> MAHHHHHHMDVGELLSYQPNRGTKRPRDDEEEEQKMRRKQTGTRERGRYREEEMTVVEEADDDKKRLLQIIDRDGEEEEEEEEPLDESSVKKMILTFEKRSYKNQELRIKFPDNPEKFMESELDLNDIIQEMHVVATMPDLYHLLVELNAVQSLLGLLGHDNTDVSIAVVDLLQELTDIDTLHESEEGAEVLIDALVDGQVVALLVQNLERLDESVKEEADGVHNTLAIVENMAEFRPEMCTEGAQQGLLQWLLKRLKAKMPFDANKLYCSEVLAILLQDNDENRELLGELDGIDVLLQQLSVFKRHNPSTAEEQEMMENLFDSLCSCLMLSSNRERFLKGEGLQLMNLMLREKKISRSSALKVLDHAMIGPEGTDNCHKFVDILGLRTIFPLFMKSPRKIKKVGTTEKEHEEHVCSILASLLRNLRGQQRTRLLNKFTENDSEKVDRLMELHFKYLGAMQVADKKIEGEKHDMVRRGEIIDNDTEEEFYLRRLDAGLFVLQHICYIMAEICNANVPQIRQRVHQILNMRGSSIKIVRHIIKEYAENIGDGRSPEFRENEQKRILGLLENF

CTNNBL1 is a spliceosome-associated protein that binds nuclear localization signals (NLSs) in splice factors CDC5L and Prp31 as well as the antibody diversifying enzyme AID. CTNNBL1 is a widely expressed, highly conserved 62 kDa nuclear protein that associates with components of the RNA splicing machinery. CTNNBL1 comprises a HEAT-like domain (including a nuclear export signal), a central armadillo domain, and a coiled-coil C-terminal domain. Our results identify CTNNBL1 as a unique selective NLS-binding protein with striking differences from karyopherin-αs.

We crystallized full-length human 6xHis-CTNNBL1 and N-terminally truncated 6xHis-CTNNBL1Δ76 (to generate a fragment that is necessary and sufficient for NLS-peptide binding). We were unable to solve the structure using molecular replacement and therefore crystallized selenomethionine-substituted protein for experimental phase determination, solving the structures of CTNNBL1Δ76 and that of full-length CTNNBL1 from crystals with the symmetry of different spacegroups. The crystals reveal the same overall structure of CTNNBL1. However, despite excellent continuity within the protein chain, we were unable to resolve any density for the N-terminal (76) amino acids in the structure of full length CTNNBL1. The N-terminus contains a disordered region and a structured HEAT-like region that includes a functional NES.> MVKLMEV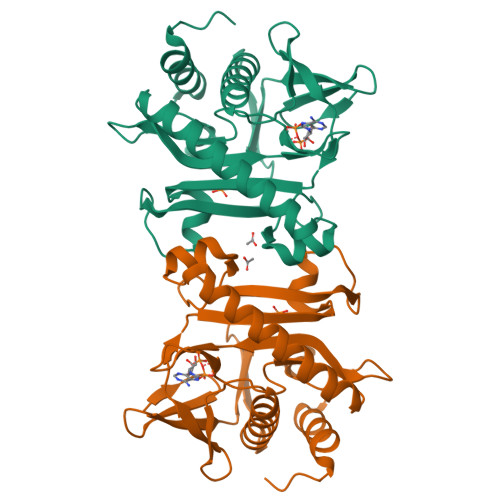YEGKAKKMIPIDDDKLIMEFKDDATAFDGTKKARFKGKGWLNAQLSVIFFKLLEEHGIKTHFIGVAGGNRLIVEKLDMYPLEVVVRNVVAGSLKKRLPLPEGYELPEPIVELYYKNDELHDPMINYYHAKVLGISLDEIKKIEEIALKVNEILKDYLAKKGIILVDFKLEFGKDKNGDIVLADEISPDTCRFWDAKTKRSLDKDVFRFDKGDLIEAYKEIYERITGEKPEF>[2x]GSHMALLVEKTTSGREYKVKDMSQADFGRLEIELAEVEMPGLMASRSEFGPSQPFKGAKITGSLHMTIQTAVLIET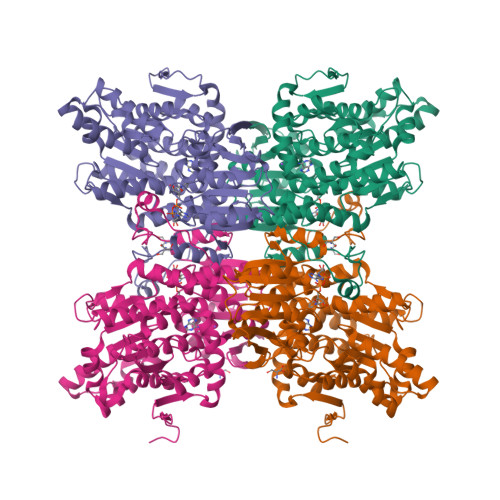LTALGAEVRWCSCNIFSTQDHAAAAIARDSAAVFAWKGETLQEYWWCTERALDWGPGGGPDLIVDDGGDTTLLIHEGVKAEEIYEKSGQFPDPDSTDNAEFKIVLSIIKEGLKTDPKRYHKMKDRVVGVSEETTTGVKRLYQMQANGTLLFPAINVNDSVTKSKFDNLYGCRHSLPDGLMRATDVMIAGKVAVVAGYGDVGKGCAAALKQAGARVIVTEIDPICALQATMEGLQVLTLEDVVSEADIFVTTTGNKDIIMLDHMKKMKNNAIVCNIGHFDNEIDMLGLETHPGVKRITIKPQTDRWVFPETNTGIIILAEGRLMNLGCATGHPSFVMSCSFTNQVIAQLELWNEKSSGKYEKKVYVLPKHLDEKVAALHLEKLGAKLTKLSKDQADYISVPVEGPYKPFHYRY> GLIVDTRDVEERVHVMRKTKLAPTVAHGVFNPEFGPAALSNKDPRLNEGVVLDEVIFSKHKSDTKMSAEDKALFRRCAADYASRLHSVLGTANAPLSIYEAIKGVDGLDAMEPDTAPGLPWALQGKRRGALIDFENGTVGPEVEAALKLMEKREYKFACQTFLKDEIRPMEKV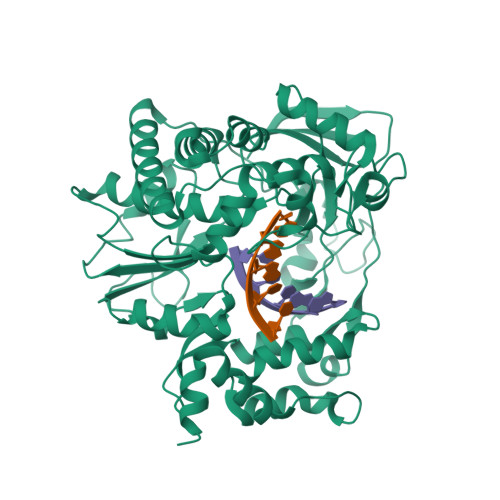RAGKTRIVDVLPVEHILYTRMMIGRFCAQMHSNNGPQIGSAVGCNPDVDWQRFGTHFAQYRNVWDVDYSAFDANHCSDAMNIMFEEVFRTEFGFHPNAEWILKTLVNTEHAYENKRITVEGGMPSGCSATSIINTILNNIYVLYALRRHYEGVELDTYTMISYGDDIVVASDYDLDFEALKPHFKSLGQTITPADKSDKGFVLGHSITDVTFLKRHFHMDYGTGFYKPVMASKTLEAILSFARRGTIQEKLISVAGLAVHSGPDEYRRLFEPFQGLFEIPSYRSLYLRWVNAVCGDAAALEHH>[2x]MSAIKPDMKIKLRMEGNVNGHHFVIDGDGTG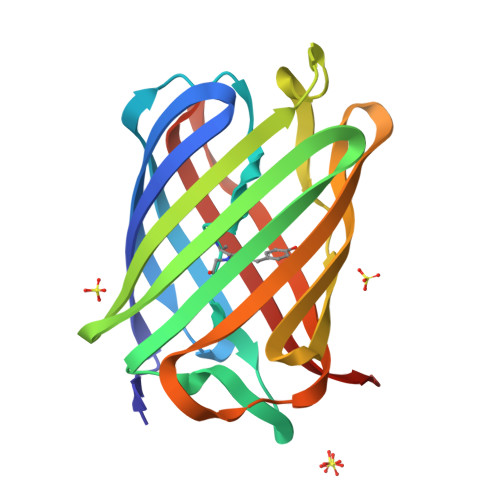KPFEGKQSMDLEVKEGGPLPFAFDILTTAFAYGNRVFAKYPDNIQDYFKQSFPKGYSWERSLTFEDGGICNARNDITMEGDTFYNKVRFYGTNFPANGPVMQKKTLKWEPSTEKMYVRDGVLTGDVETALLLEGNAHYRCDFRTTYKAKEKGVKLPGAHFVDHCIEILSHDKDYNKVKLYEHAVAHSGLPN>[2x]MTSETTTTPSRVPQTANDLLARRYATIGPHSPLFYRQPLELVSGSGVWLTDAQGKVYLDGYNNVPHVGHANPAVADAIYQQLLTVNLHTRYLNSRVVEYAEALLSKFDGALERLFLTNSGSEANELALRIARQHTGNTGVLVSDFSYHGNTTSLAEITTGLTVHEPLGAHVRALRIPDVSGIAEVDVPVLLEQSLADVDAAIASLQAAGHGVSVFLFDPLFSTEGLLQLPSGYIEGVATRVRAAGGLVI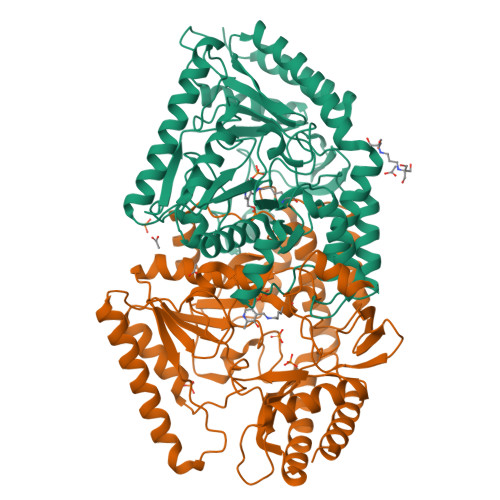SDEVQSGFGRTGSGMWGYQMFNVEPELVTMGKPMGNGHPIGAVVTTAELLDEFGRHNMFFNTFAGNPVSSAAGLAVLRYMDQEDLMAKADQLGKYIRKRLENIAQRSGNVGSVRGRGLFFGIDIIESDGSRNPAPALTKILIEDMRERGVLISRVGPHDNVLKMRPPLVFGREHADILLGQLELSLASLPQPGNLVL>MGSKCSNSGIECDSSGTCINPSNWCDGVSHCPGGEDENRCVRLYGPNFILQVYSSQRKSWHPVCQDDWNENYGRAACRDMGYKNNFYSSQGIVDDSGSTSFMKLNTSAGNVDIYKKLYHSDACSSKAVVSLRCIACGVNLNDDDDK[2x];>[2x]IVGGESALPGAWPWQVSLHVQNVHVCGGSIITPEWIVTAAHCVEKPLNNPWHWTAFAGILRQSFMFYGAGYQVEKVISHPNYDSKTKNNDIALMKLQKPLTFNDLVKPVCLPNPGMMLQPEQLCWISGWGATEEKGKTSEVLNAAKVLLIETQRCNSRYVYDNLITPAMICAGFLQGNVDSCQGDSGGPLVTSKNNIWWLIGDTSWGSGCAKAYRPGVYGNVMVFTDWIYRQMRADGEFVEHHHHHHHH

Host proteases, TMPRSS2 and CTSL/CTSB cleave the SARS-CoV-2 spike to play a crucial role in the two alternative pathways of viral entry and are characterized as promising pharmacological targets. The entry of SARS-CoV-2 depends on two distinctive pathways, cell surface entry and endosomal entry, where the transmembrane serine protease, TMPRSS2, and endosomal cysteine proteases cathepsin L/B (CTSL/CTSB) cleave the viral spike protein. The crystal structures of TMPRSS2 and CTSL/CTSB in complex with the potent inhibitors were determined to reveal their specific mode of interaction.

In light of the crystal structures of K777 and nafamostat complexed with their respective proteases, we devised a bispecific compound, named 212-148. An ethyl linker was utilized to construct this bispecific compound by connecting the pharmacophoric groups of K777 and nafamostat. As expected, 212-148 not only showed potent inhibition for CTSL/CTSB with respective IC50 values of 2.13 and 64.07 nM but also suppressed TMPRSS2 enzymatic activity with an IC50 value of 1.38 μM. Further, 212-148 demonstrated effective inhibition of SARS-CoV-2 Delta variant spike protein cleavage in vitro, albeit with a decreased anti-TMPRSS2 inhibitory potency. Further structural studies showed that 212-148 covalently linked to the TMPRSS2 catalytic site with guanidinobenzoyl moiety at the post-reaction state, the same as nafamostat and camostat. The ester group in their common guanidinobenzoyl moiety then reacts with the catalytic serine of TMPRSS2 to form the acyl-enzyme intermediate and cleave off the “leaving group”. The guanidinobenzoyl group stays covalently linked to the catalytic serine and disables the protease activity. In Calu-3 cells, 212-148 inhibits the SARS-CoV-2 Omicron BA.2 and Delta variants infection with EC50 values of 64.4 (SI = 5,391) and 235.2 nM (SI = 1,476), respectively. Although its anti-TMPRSS2 inhibitory activity decreased in comparison to nafamostat, 212-148 showed nanomolar potency against Omicron and Delta variants while maintaining good cell viability.>[4x]SITENTSWNKEFSAEAVNGVFVLCKSSSKSCATNDLARASKEYLPASTFKIPNAIIGLETGVIKNEHQVFKWDGKPRAMKQWERDLTLRGAIQVSAVPVFQQIAREV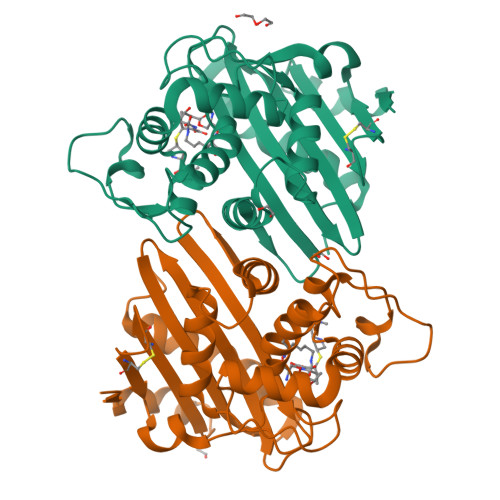GEVRMQKYLKKFSYGNQNISGGIDKFWLEGQLRISAVNQVEFLESLYLNKLSASKENQLIVKEALVTEAAPEYLVHSKTGWGMGVTPQVGWWVGWVEKETEVYFFAFNMDIDNESKLPLRKSIPTKIMESEGIIGG> GSHMANLDRTDDLVYLNVMELVRAVLELKNELSQLPPEGYVVVVKNVGLTLRKLIGSVDDLLPSLPSSSRTEIEGTQKLLNKDLAELINKMRLAQQNAVTSLSEEAKRQMLTASHTLAVDAKNLLDAVDQAKVLANLAH;> KTSAAAQLD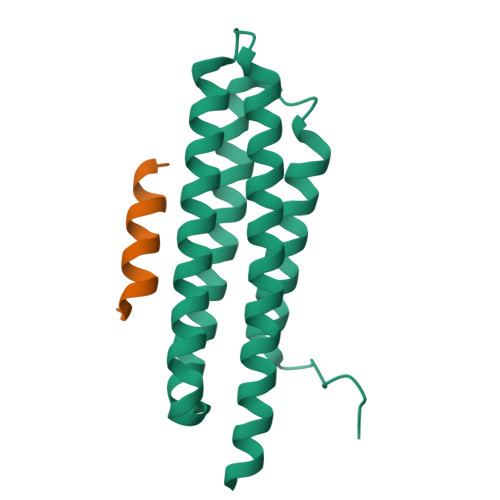ELMAHLTEMQ>MKIRDLLKARRGPLFSFEFFPPKDPEGEEALFRTLEELKAFRPAFVSITYGAMGSTRERSVAWAQRIQSLGLNPLAHLTVAGQSRKEVAEVLHRFVESGVENLLALRGDPPRGERVFRPHPEGFRYAAELVALIRERYGDRVSVGGAAYPEGHPESESLEADLRHFKAKVEAGLDFAITQLFFNNAHYFGFLERARRAGIGIPILPGIMPVTSYRQLRRFTEVCGASIPGPLLAKLERHQDDPKAVLEIGVEHAVRQVAELLEAGVEGVHFYTLNKSPATRMVLERLGLRPASGQP[2x]

The flavoprotein methylenetetrahydrofolate reductase (MTHFR) catalyzes the reduction of N5, N10-methylenetetrahydrofolate (CH2-H4folate) to N5-methyltetrahydrofolate (CH3-H4folate), committing a methyl group from the folate cycle to the methionine one. MTHFR requires flavin adenine nucleotide (FAD) as a noncovalently bound cofactor, which acts as an intermediary electron shuttle. All MTHFRs share a highly conserved catalytic domain, despite varying oligomerization states, such as a dimer in Thermus thermophilus HB8 (tMTHFR) versus a tetramer in Escherichia coli (eMTHFR). All MTHFR catalytic domains share the same β8α8 barrel topology, a typical triose phosphate isomerase barrel structure.

In the absence of folate, two different FAD-bound tMTHFR structures with different intermonomer interfaces have been described. In one of the structures, only one active site in the dimer is occupied by FAD (half-FAD occupancy, dimer mode 1) while both active sites are occupied in the other (full-FAD occupancy, dimer mode 2). It is worth noting that tMTHFR purifies in the half-FAD occupancy state; only the addition of excess FAD leads to the observance of the full-FAD occupancy state. In contrast, in the folate-free tMTHFR structure, the distance between Thr and Glu is found to be 5.7 Å, suggesting that the triad expansion to include the interacting Thr49 and formation of a tetrad is triggered or is coupled to binding of a specific folate form. Indeed, the Thr coordination in the folate-free tMTHFR structure is very similar to that in the eMTHFR structure with or without CH3-H4folate. It has to be noted that while the Thr residue exhibits a dynamic behavior, the positions of the Ser, His, and Glu residues in the triad remain largely unchanged.> SNASDTRKAIDTISNLLKI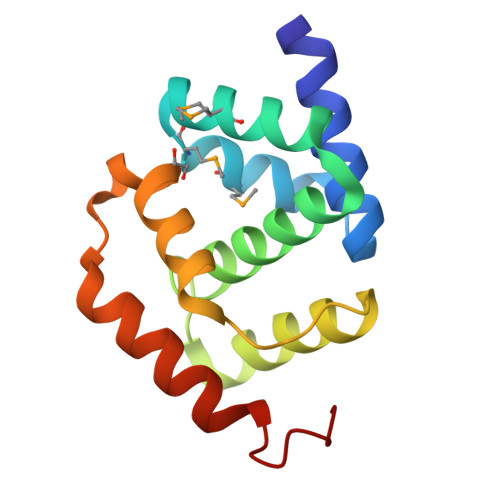KPIYIESMLQEMGPRQTQMFIRSTSNGSAEEVRKAAYLVFIYHTFIKNPSDENVELWRNTLIRAQISPILAAEHTDAALFYFAELDLDAFELAQFRRHYNLHFNPEPGTLLH>GGCGCGAGGAAGGAGGUCUGAGGAGGUCACUGCGCC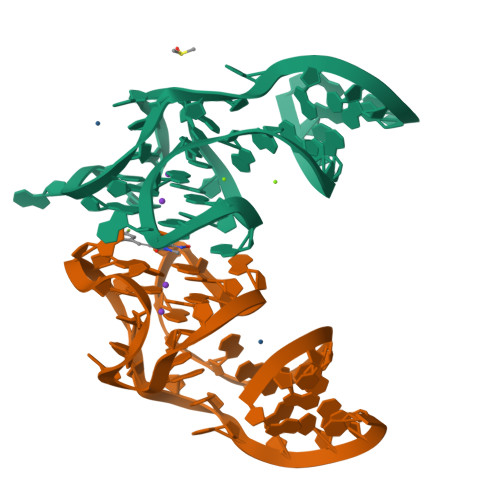[2x]In 2011, desmoglein-2 (DSG2), a component of desmosomes carrying four extracellular domains (EC1 to EC4) has been reported to be the main receptor of HAdV of serotype 3, 7, 11, and 14. The critical entry step in the viral cycle is mediated by the adenovirus trimeric fiber and more especially by its distal globular domain called the ‘knob’. In the present study, we investigate the binding mechanism of the ARD causing agent HAdV7 to the EC23 module of DSG2 using biochemical and biophysical methods. We report the atomic structure of the complex solved by cryo-EM using phase-plate providing improved high-contrast images.

The trimeric HAd7K appears decorated with variable amount of extra densities confirming that the complex between HAd7K and EC23 might have a variable stoichiometry under the conditions used for cryo-EM. Extensive 3D classifications and refinements indeed show that the complex mainly exists in two forms, i.e., a HAd7K trimer can interact with two or three EC23 modules hereafter named HAd7K-(EC23)2 and HAd7K-(EC23)3, respectively. There are 40% more particles in the final 3D reconstruction of HAd7K-(EC23)2 than in the one of HAd7K-(EC23)3. According to that statistics, it follows that the main stoichiometry of the complex by cryo-EM is two EC23 modules per HAd7K trimer. HAd7K-(EC23)2 and HAd7K-(EC23)3 were solved to 3.5 and 3.1 Å resolution, respectively, which allowed the fitting and refinement of two atomic models using the existing X-ray structures of HAd7K and EC23. The overall root mean square deviation (RMSD) between HAd7K-(EC23)2 and HAd7K-(EC23)3 (without the third EC23 module) is 0.5 Å. Each EC23 module interacts with two different monomers of the HAd7K. Furthermore, each EC domain (i.e., EC2 or EC3) interacts with one HAd7K monomer. A small loop in the EC2 domain which contains residues S175 and T177 interacts with a β strand of HAd7K through putative hydrogen bonds with N190 and N192. For the EC3 domain, the main interacting residue is R316 which fits into a pocket formed by two loops at the surface of one HAd7K monomer.

>[3x]GSHMGLTFNSNNICIDDNINTLWTGVNPTTANCQIMASSESNDCKLILTLVKTGALVTAFVYVIGVSNDFNMLTTHKNINFTAELFFDSTGNLLTSLSSLKTPLNHKSGQNMATGALTNAKGFMPSTTAYPFNVNSREKENYIYGTCYYTASDHTAFPIDISVMLNQRALNNETSYCIRVTWSWNTGVAPEVQTSATTLVTSPFTFYYIREDD;>[2x]QGAMEVLDINDNEPVFTQDVFVGSVEELSAAHTLVMKINATDADEPNTLNSKISYRIVSLEPAYPPVFYLNKDTGEIYTTSVTLDREEHSSYTLTVEARDGNGEVTDKPVKQAQVQIRILDVNDNIPVVENKVLEGMVEENQVNVEVTRIKVFDADEIGSDNWLANFTFASGNEGGYFHIETDAQTNEGIVTLIKEVDYEEMKNLDFSVIVANKAAFHKSIRSKYKPTPIPIKVKVKNVKEGI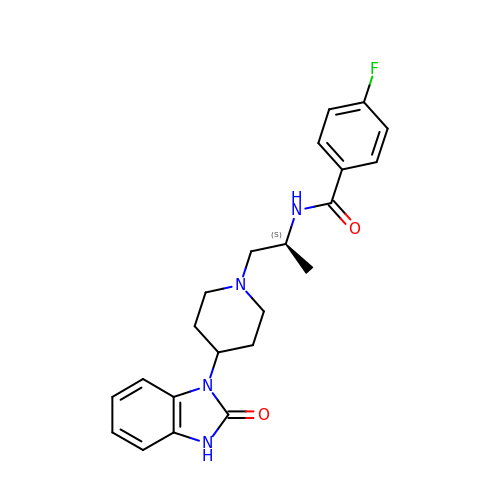4-fluoro-N-{(2S)-1-[4-(2-oxo-2,3-dihydro-1H-benzimidazol-1-yl)piperidin-1-yl]propan-2-yl}benzamide | C22 H25 F N4 O2 | KKKBWVASRHMJPO-HNNXBMFYSA-N> MGKSREQTMENI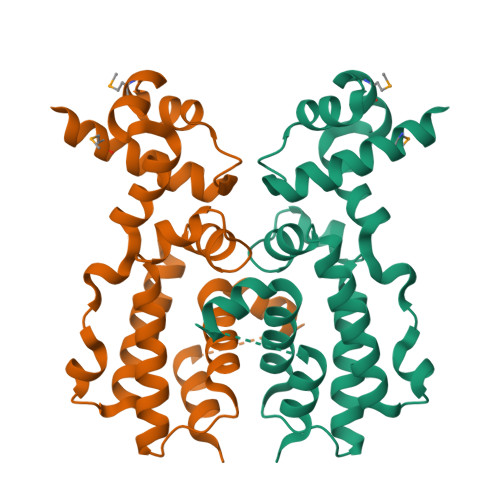LKAAKKKFGERGYEGTSIQEIAKEAKVNVAMASYYFNGKENLYYEVFKKYGLANELPNFLEKNQFNPINALREYLTVFTTHIKENPEIGTLAYEEIIKESARLEKIKPYFIGSFEQLKEILQEGEKQGVFHFFSINHTIHWITSIVLFPKFKKFIDSLGTNETNDTNHEWMPEDLVSRIISALTDKPNI2-[(1S)-1-BENZYL-2-SULFANYLETHYL]-1H-IMIDAZO[4,5-C]PYRIDIN-5-IUM 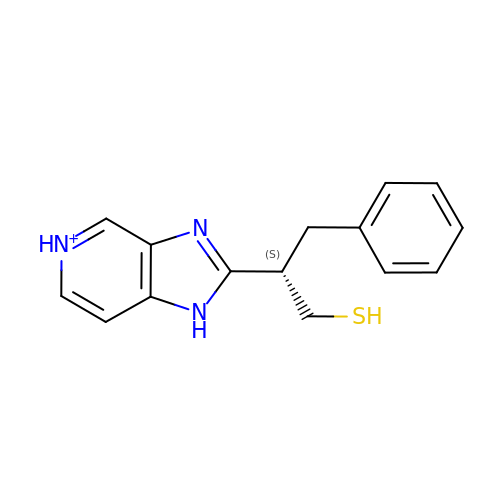| C15 H16 N3 S | DCUCDCAIOMIBEA-GFCCVEGCSA-O>KPNILIIMVDQLNGKLFPDGPADFLHAPNLKALAKRSARFHNNYTSSPLAAPARASFMAGQLPSRTRVYDNAAEYQSSIPTYAHHLRRAGYYTALSGKMHLVGPDQLHGFEERLTTDIYPADFGWTPDYRKPGERIDWWYHNLGSVTGAGVAEITNQMEYDDEVAFLANQKLYQLSRENDDESRRPWCLTVSFTHPHDPYVARRKFWDLYEDCEHLTPEVGAIPLDEQDPHSQRIMLSCDYQNFDVTEENVRRSRRAYFANISYLDEKVGELIDTLTRTRMLDDTLILFCSDHGDMLGERGLWFKMNFFEGSARVPLMIAGPGIAPGLHLTPTSNLDVTPTLADLAGISLEEVRPWTDGVSLVPMVNGVERTEPVLMEYAAEASYAPLVAIREGKWKYVYCALDPEQLFDLEADPLELTNLAENPRGPVDQATLTAFRDMRAAHWDMEAFDAAVRESQARRWVVYEALRNGAYYPWDHQPLQKASERYMRNHMNLDTLEESKRYPRGE[4x]

Choline-O-sulfatase (COSe; EC 3.1.6.6) is a member of the alkaline phosphatase (AP) superfamily, and its natural function is to hydrolyze choline-O-sulfate into choline and sulfate. Choline-O-sulfatase (COSe; EC 3.1.6.6) is responsible for the first step of this pathway, consisting of the breakdown of COS into choline. This enzyme belongs to the S1 family of sulfatases (subfamily 12) according to the SulfAtlas database. Like other arylsulfatases and phosphonate monoester hydrolases (PMHs; van Loo et al., 2010, van Loo, Bayer et al., 2019), SmeCOse is a mononuclear metalloenzyme. DLS experiments performed at pH 8.0 show a single peak in the particle-size distribution by intensity, with a hydrodynamic radius of 5.7 ± 2.1 nm, which corresponds to a globular protein size of 200 kDa, also supporting a tetrameric quaternary arrangement.

The COSe from S. meliloti CECT4857 used in this work presents a single L105F mutation with respect to that protein (Genbank Accession No. QAT12853). WT SmeCOSe crystals alone or co-crystallized with choline were grown in 1.0 M Li2SO4, 0.1 M Tris pH 7.0, whereas the HEPES-bound C54S SmeCOSe structure was obtained from crystals obtained using 1.5 M Li2SO4, 0.1 M HEPES pH 7.5; they belonged to space group C121. Whereas the presence of this PTM had already been ascertained, inspection of the catalytic environment of the WT SmeCOSe structure clearly shows densities shaping a hydrated formylglycine (FGly) residue. Based on other studies showing the necessity of high sulfate concentrations to inhibit hydrolytic sulfatases, we used concentrations of sulfate of up to 200 mM to conduct TSA experiments with SmeCOSe, showing a of 0.8°C. On the other hand, only higher concentrations of ammonium sulfate (up to 500 mM) produced a slight decrease (a 15% decrease) in SmeCOSe activity. A sulfate molecule could be modeled into the catalytic center of the WT SmeCOSe structure, most likely arising from the high concentrations of sulfate used in the crystallization conditions (1 M ammonium sulfate). In the four chains modeled in this structure, Asn75 is at a distance between 2.8 and 3.1 Å from the sulfate ion; this residue occupies similar positions to Asn73 in Rhizobium leguminosarum PMH and Arg166 in E. coli AP, with the latter being reported to coordinate the substrate, the intermediate and the products of the reaction. However, our structures do not support this hypothesis, since Lys102 is at a distance of more than 4.0 Å in our sulfate-bound and HEPES-bound structures. Nonetheless, Lys102 is at a binding distance to FGly54 in this structure and might assist during FGly regeneration (see below).Pol μ is capable of performing gap-filling repair synthesis in the nonhomologous end joining (NHEJ) pathway. Compared with replicative DNA polymerase, Pol μ lacks proofreading activity, with an intrinsically high error rate of 10−3–10−5 for dNTP incorporation. Here, crystal structures and kinetics of Pol μ substituting dGTP for dATP on gapped DNA substrates containing templating T were determined and compared.

To investigate the mechanism of dGTP misincorporation on 1-nt gapped DNA, we first solved the binary structure of Pol μ:DNA. This binary complex with template T is almost identical to the published Pol μ:DNA binary complex containing templating A (PDB ID: 4LZG29), except for the interactions of the templating base in the active site. By replacing dA with dT, the templating T interacts snugly with Lys438 and Gln441, which adopts rotamer conformations similar to those observed in the Complex 1 structure. The space between templating T and thumb domain is filled with water and glycerol molecules. Gln441 from minor groove interacts with templating T in our binary complex and undergoes a rotamer change to avoid clashes with incoming nucleotides regardless of whether correct insertion or misincorporation occurred. Gln441 interacts with the unpaired 5ʹ templating T in both binary complex and Complex 1 structures and undergoes a rotamer change toward the finger domain to avoid clashes with base-pairing after incoming nucleotide binding, which is observed in all the normal and misincorporation ternary structures solved by our group and others.

> MLPKRRRARVGSPSGDAASSTPPSTRFPGVAIYLVEPRMGRSRRAFLTGLARSKGFRVLDACSSEATHVVMEETSAEEAVSWQERRMAAAPPGCTPPALLDISWLTESLGAGQPVPVECRHRLEVAGPRKGPLSPAWMPAYACQRPTPLTHHNTGLSEALEILAEAAGFEGSEGRLLTFCRAASVLKALPSPVTTLSQLQGLPHFGEHSSRVVQELLEHGVCEEVERVRRSERYQTMKLFTQIFGVGVKTADRWYREGLRTLDDLREQPQKLTQQQKAGLQHHQDLSTPVLRSDVDALQQVVEEAVGQALPGATVTLTGGFRRGKLQGHDVDFLITHPKEGQEAGLLPRVMCRLQDQGLILYHQHQHSCCESPTRLAQQSHMDAFERSFCIFRLPQPGSWKAVRVDLVVAPVSQFPFALLGWTGSKLFQRELRRFSRKEKGLWLNSHGLFDPEQKTFFQAASEEDIFRHLGLEYLPPEQRNA> MPYSVGFREADAATSFLRAARSGNLDKALDHLRNGVDINTCNQNGLNGLHLASKEGHVKMVVELLHKEIILETTTKKGNTALHIAALAGQDEVVRELVNYGANVNAQSQKGFTPLYMAAQENH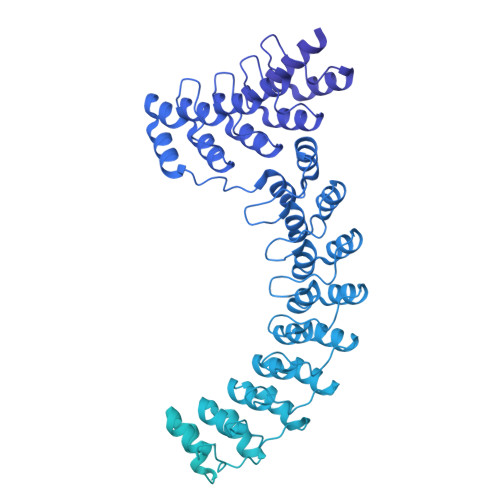LEVVKFLLENGANQNVATEDGFTPLAVALQQGHENVVAHLINYGTKGKVRLPALHIAARNDDTRTAAVLLQNDPNPDVLSKTGFTPLHIAAHYENLNVAQLLLNRGASVNFTPQNGITPLHIASRRGNVIMVRLLLDRGAQIETKTKDELTPLHCAARNGHVRISEILLDHGAPIQAKTKNGLSPIHMAAQGDHLDCVRLLLQYDAEIDDITLDHLTPLHVAAHCGHHRVAKVLLDKGAKPNSRALNGFTPLHIACKKNHVRVMELLLKTGASIDAVTESGLTPLHVASFMGHLPIVKNLLQRGASPNVSNVKVETPLHMAARAGHTEVAKYLLQNKAKVNAKAKDDQTPLHCAARIGHTNMVKLLLENNANPNLATTAGHTPLHIAAREGHVETVLALLEKEASQACMTKKGFTPLHVAAKYGKVRVAELLLERDAHPNAAGKNGLTPLHVAVHHNNLDIVKLLLPRGGSPHSPAWNGYTPLHIAAKQNQVEVARSLLQYGGSANAESVQGVTPLHLAAQEGHAEMVALLLSKQANGNLGNKSGLTPLHLVAQEGHVPVADVLIKHGVMVDATTRMGYTPLHVASHYGNIKLVKFLLQHQADVNAKTKLGYSPLHQAAQQGHTDIVTLLLKNGASPNEVSSDGTTPLAIAKRLGYISVTDVLKVVTDETSFVLVSDKHRMSFPETVDEILDVSEDEGEELISFKAERRDSRDVDEEKELLDFVPKLDQVVESPAIPRIPCAMPETVVIRSEEQEQASKEYDEDSLIPSSPATETSDNISPVASPVHTGFLVSFMVDARGGSMRGSRHNGLRVVIPPRTCAAPTRITCRLVKPQKLSTPPPLAEEEGLASRIIALGPTGAQFLSPVIVEIPHFASHGRGDRELVVLRSENGSVWKEHRSRYGESYLDQILNGMDEELGSLEELEKKRVCRIITTDFPLYFVIMSRLCQDYDTIGPEGGSLKSKLVPLVQATFPENAVTKRVKLALQAQPVPDELVTKLLGNQATFSPIVTVEPRRRKFHRPIGLRIPLPPSWTDNPRDSGEGDTTSLRLLCSVIGGTDQAQWEDITGTTKLVYANECANFTTNVSARFWLSDCPRTAEAVNFATLLYKELTAVPYMAKFVIFAKMNDPREGRLRCYCMTDDKVDKTLEQHENFVEVARSRDIEVLEGMSLFAELSGNLVPVKKAAQQRSFHFQSFRENRLAMPVKVRDSSREPGGSLSFLRKAMKYEDTQHILCHLNITMPPCAKGSGAEDRRRTPTPLALRYSILSESTPGSLSGTEQAEMKMAVISEHLGLSWAELARELQFSVEDINRIRVENPNSLLEQSVALLNLWVIREGQNANMENLYTALQSIDRGEIVNMLEGSGRQSRNLKPDRRHTDRDYSLSPSQMNGYSSLQDELLSPASLGCALSSPLRADQYWNEVAVLDAIPLAATEHDTMLEMSDMQVWSAGLTPSLVTAEDSSLECSKAEDSDATGHEWKLEGALSEEPRGPELGSLELVEDDTVDSDATNGLIDLLEQEEGQRSEEKLPGSKRQDDATGAGQDSENEVSLVSGHQRGQARITHSPTVSQVTERSQDRLQDWDADGSIVSYLQDAAQGSWQEEVTQGPHSFQGTSTMTEGLEPGGSQEYEKVLVSVSEHTWTEQPEAESSQADRDRRQQGQEEQVQEAKNTFTQVVQGNEFQNIPGEQVTEEQFTDEQGNIVTKKIIRKVVRQIDLSSADAAQEHEEVTVEGPLEDPSELEVDIDYFMKHSKDHTSTPNP>MLPKLVITHRVHEEILQLLAPHCELITNQTDSTLTREEILRRCRDAQAMMAFMPDRVDADFLQACPELRVIGCALKGFDNFDVDACTARGVWLTFVPDLLTVPTAELAIGLAVGLGRHLRAADAFVRSGKFRGWQPRFYGTGLDNATVGFLGMGAIGLAMADRLQGWGATLQYHEAKALDTQTEQRLGLRQVACSELFASSDFILLALPLNADTLHLVNAELLALV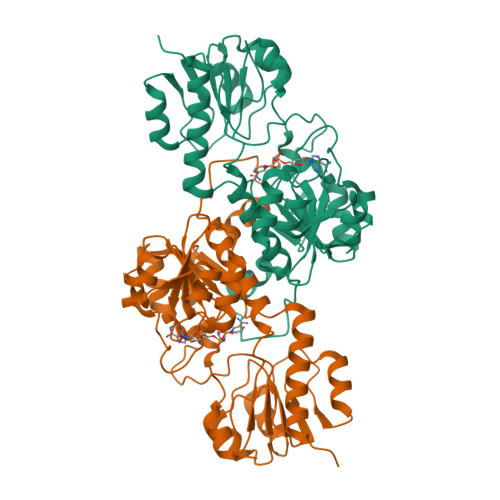RPGALLVNPCRGSVVDEAAVLAALERGQLGGYAADVFEMEDWARADRPQQIDPALLAHPNTLFTPHIGSAVRAVRLEIERCAAQNILQALAGERPINAVNRLPK[8x]> MTDLSSLIETADLRLLLTTVPTETEALYLALAAVEKGLAAEVLITPVTRVRRENGKLVVEDVYRL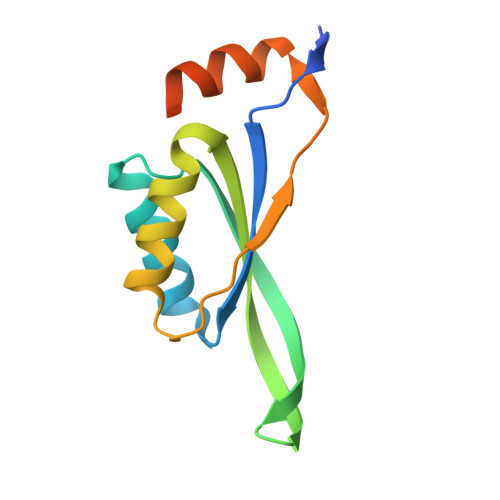SFKTTRERLDALVAWLQRRHPLALPECLVLTPIASSVAYRDWLRSSLQGGSHHWGGHHHHHH>[6x]MF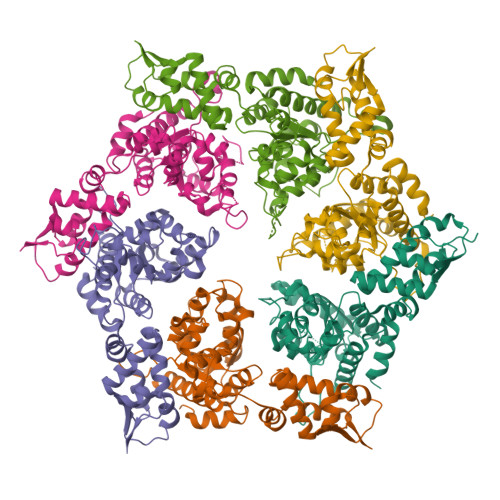KFNDEKVQLKCSFCGKTQDQVRKLVAGPGVYICDECIELCNEIIEEELGISEFVDFGEVPKPQEIRHILSDYVIGQERAKKALAVAVYNHYKRINSNETKEDEVELSKSNICLIGPTGSGKTLLAQTLARILNVPFAIADATSLTEAGYVGEDVENILLKLIQSADYDVEKAEKGIIYIDQIDKVARKSENPSITRDVSGEGVQQALLKILEGTVASVPPQGGRKHPHQELIQIDTGNILFIVGGAFDGIEQIVKNRMGEKVIGFGTDNAKLKDDETYLSRVVPEDLLKFGLIPEFIGRLPVIATLEQLDEAALVSILTEPKNALVKQYKRMLELDDVELEFEPTALIEIAKEAIERKTGARGLRSIIEQIMLEVMFEIPSRDDITKCIITEKAARGEEEPQLQLEDGSIIPIKTSA> GSSGSSGMIKEYRTIKEVVGPLMAVEKVSGVKYEELIEVRMQNGEIRRGQVLEVQEDKAMVQIFEGTSGICLKNSSVRFLGHPLQLGVSEDMIGRVFDGLGRPKDNGPEILPEKYLDINGEVINPIARDYPDEFIQTGISAIDHLNTLVRGQKLPVFSGSGLPHKELAAQIARQATVLDSSDDFAVVFAAIGITFEEAEFFMEDFRQTGAIDRSVMFMNLANDPAIERIATPRMALTAAEYLAYEKGMHVLV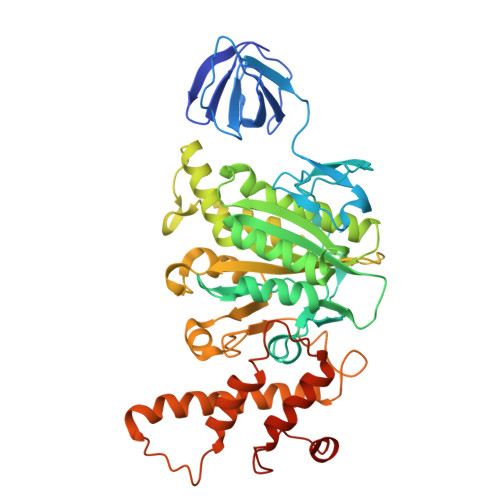IMTDMTNYAEALREISAARREVPGRRGYPGYLYTNLATLFERAGRIRGLKGSVTQIPILTMPEDDKTHPIPDLTGYITEGQIILTRELYKSGIQPPIDVLPSLSRLKDKGTGAGKTREDHAATMNQLFAAYAQGKQAKELAVVLGESALSDIDKIYAKFAERFENEYVNQGFYTNRTITETLDLGWELLAMLPRTELKRIKDDLLDKYLPEGK>MHHHHHHGSPLPATHDLHISGSINGHEFDLEGSGKGNAKEGYQELHLKSNKGDLSFSPWILVPNIGYGFYQYLPFPDGAMSPYQAAMHDGSGYVMHRSMQFEDGAMLHSDHRYIYKGNHIKGEFRLTGSGFPADGPVMTNSLTAADWCVDKLL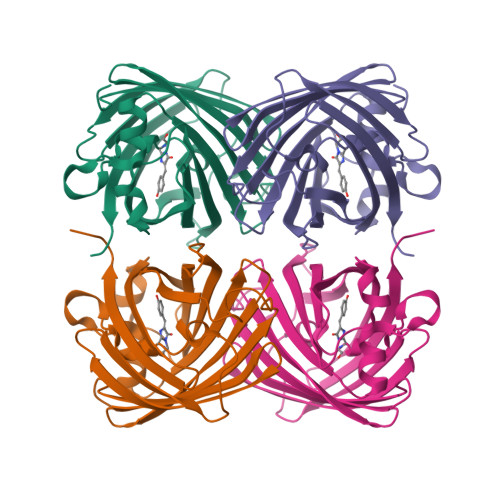YPNDNTIIGKFDWTYTTTSGKRYQSDVQTNVTFGKPIAADILKKQPMFVFRKVELKHTKTELNFKQWQKAFQDIA[2x]1-[3-[(4~{S})-6-azanyl-5-cyano-3-methyl-4-propan-2-yl-2~{H}-pyrano[2,3-c]pyrazol-4-yl]-5-fluoranyl-phenyl]piperidine-4-carboxylic 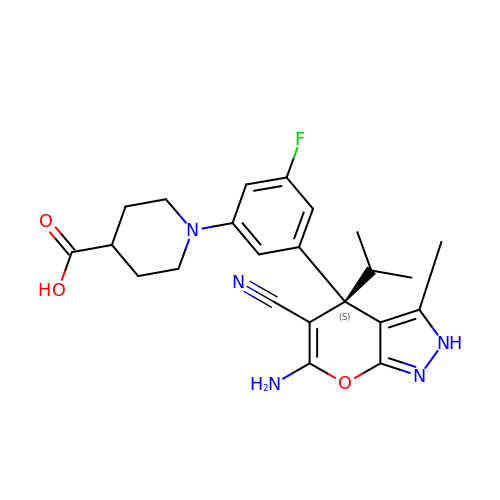acid | C23 H26 F N5 O3 | JPUKBKCOTBHVDC-QHCPKHFHSA-N> ASPQLEELITKVSKAHQETFPSLCQLGKYTTNSSADHRVQLDLGLWDKFSELATKCIIKIVEFAKRLPGFTGLSIADQITLLKAACLDILMLRICTRYTPEQDTMTFSDGLTLNRTQMHNAGFGPLTDLVFAFAGQLLPL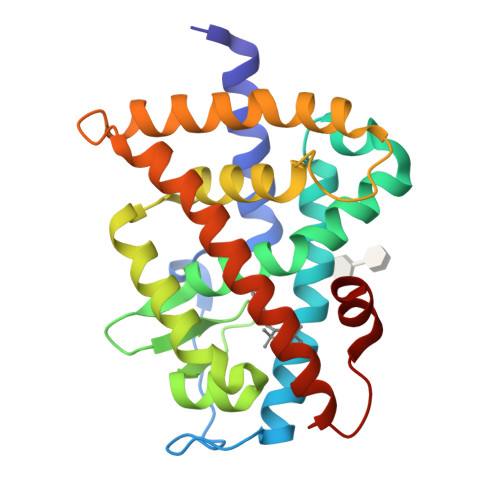EMDDTETGLLSAICLICGDRMDLEEPEKVDKLQEPLLEALRLYARRRRPSQPYMFPRMLMKITDLRGISTKGAERAITLKMEIPGPMPPLIREMLE>SMRPQPGDGERRYREASARKKIRLDRKYIVSCKQTEVPLSVPWDPSNQVYLSYNNVSSLKMLVAKDNWVLSSEISQVRLYTLEDDKFLSFHMEMVVHVDAAQAFLLLSDLRQRPEWDKHYRSVELVQQVDEDDAIYHVTSPALGGHTKPQDFVILASRRKPCDNGDPYVIALRSVTLPTHR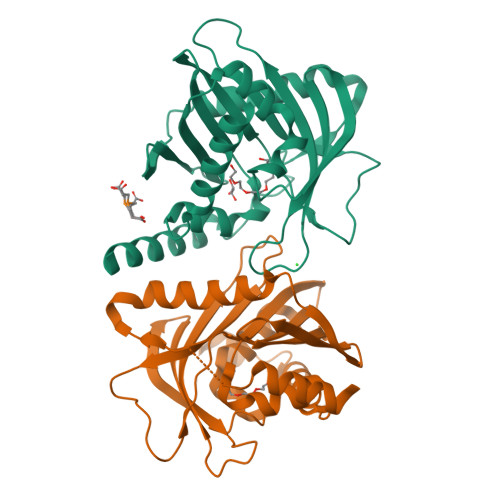ETPEYRRGETLCSGFCLWREGDQLTKVSYYNQATPGVLNYVTTNVAGLSSEFYTTFKACEQFLLDNRNDLAPSLQTL[2x]> MDVSFRLSGATSSSYGVFISNLRKALPNERKLYDIPLLRSSLPGSQRYALIHLTNYADETISVAIDVTNVYIMGYRAGDTSYFFNQASATEAAKYVFKDAMRKVTLPYSGNYERLQTAAGKIRENIPLGLPALDSAITTLFYYNANSAASALMVLI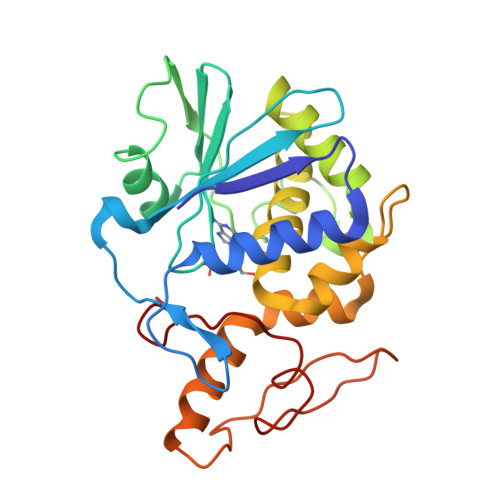QSTSEAARYKFIEQQIGKRVDKTFLPSLAIISLENSWSALSKQIQIASTNNGQFESPVVLINAQNQRVTITNVDAGVVTSNIALLLNRNNMA> GPEVQKPLHEQLWYHGAIPRAEVAELLVHSGDFLVRESQGKQEYVLSVLWDGLPRHFIIQSLDNLYRLEGEGFPSIPLLIDHLLSTQQPLTKKSGVVLHRAVPKDKWVLNHEDLVLGEQIGRGNFGEVFSGRLRADNTLVAVKSCRETLPPDLKAKFLQ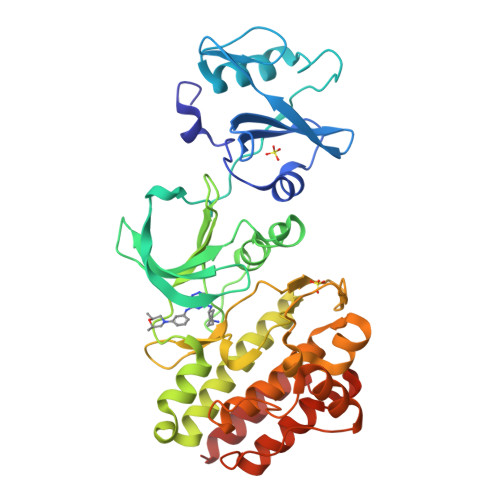EARILKQYSHPNIVRLIGVCTQKQPIYIVMELVQGGDFLTFLRTEGARLRVKTLLEMVGDAAAGMEYLESKCCIHRDLAARNCLVTEKNVLKISDFGMSREEADGVYAASGGLRQVPVKWTAPEALNYGRYSSESDVWSFGILLWETFSLGASPYPNLSNQQTREFVEKGGRLPCPELCPDAVFRLMEQCWAYEPGQRPSFSTIYQELQSIRKRHR>[2x]MTALEVLGGWPVPAAAAAVIGPAGVLATHGDTA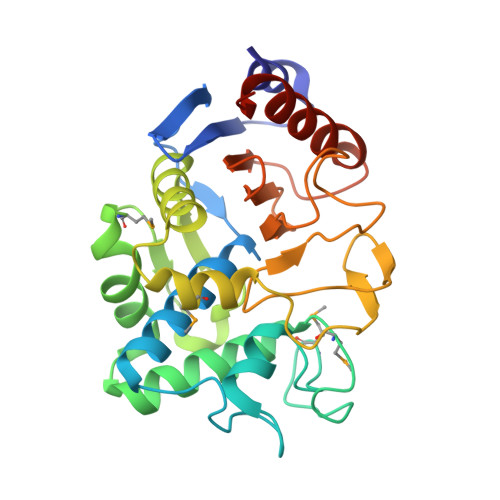RVFALASVTKPLVARAAQVAVEEGVVNLDTPAGPPGSTVRHLLAHTSGLAMHSDQALARPGTRRMYSNYGFTVLAESVQRESGIEFGRYLTEAVCEPLGMVTTRLDGGPAAAGFGATSTVADLAVFAGDLLRPSTVSAQMHADATTVQFPGLDGVLPGYGVQRPNDWGLGFEIRNSKSPHWTGECNSTRTFGHFGQSGGFIWVDPKADLALVVLTARDFGDWALDLWPAISDAVLAEYTLEHHHHHH>ATSDSNMLLNYVPVYVMLPLGVVNVDNVFEDPDGLKEQLLQLRAAGVDGVMVDVWWGIIELKGPKQYDWRAYRSLLQLVQECGLTLQAIMSFHQCGGNVGDIVNIPIPQWVLDIGESNHDIFYTNRSGTRNKEYLTVGVDNEPIFHGRTAIEIYSDYMKSFRENMSDFLESGLIIDIEVGLGPAGELRYPSYPQSQGWEFPGIGEFQCYDKYLKADFKAAVARAGHPEWELPDDAGKYNDVPESTGFFKSNGTYVTEKGKFFLTWYSNKLLNHGDQILDEANKAFLGCKVKLAIKVSGIHWWYKVENHAAELTAGYYNLNDRDGYRPIARMLSRHHAILNFTCLEMRDSEQPSDAKSGPQELVQQVLSGGWREYIRVAGENALPRYDATAYNQIIL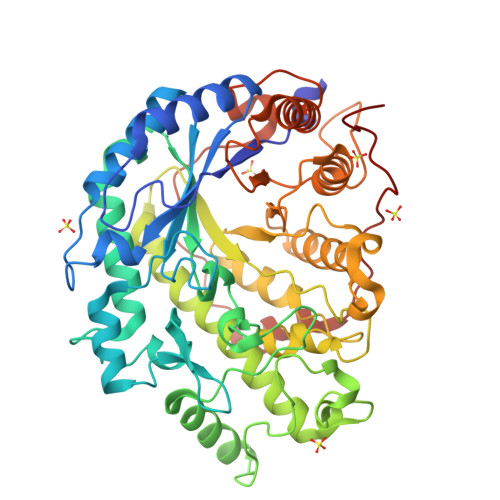NARPQGVNNNGPPKLSMFGVTYLRLSDDLLQKSNFNIFKKFVLKMHADQDYCANPQKYNHAITPLSPSAPKIPIEVLLEATKPTRPFPWLDETDMKVDG[4x]> SMASKNNIFNKYPTIIHGEARGENDEFVVHTRYPRFLARKSFDDNFTGEMPAKPVNGELGQIGEPRRLAYDSRLGLWLSDFIMLDNNKPKNMEDWLGQLKA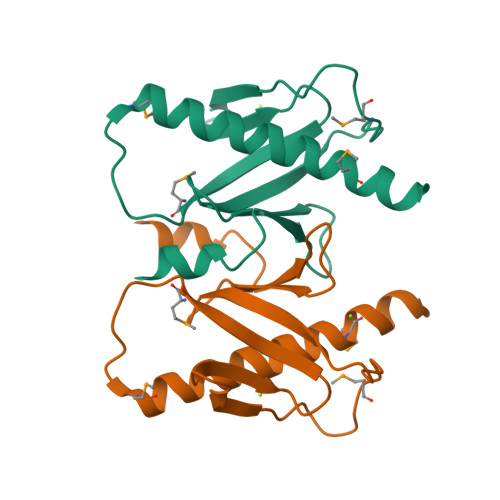ACDRIAADDLMLNEDAADLEGWDD>SNASDKGKLSLQDVAELIRARACQRVVVMVGAGISTPSGIPDFRSPGSGLYSNLQQYDLPYPEAIFELPFFFHNPKPFFTLAKELYPGNYKPNVTHYFLRLLHDKGLLLR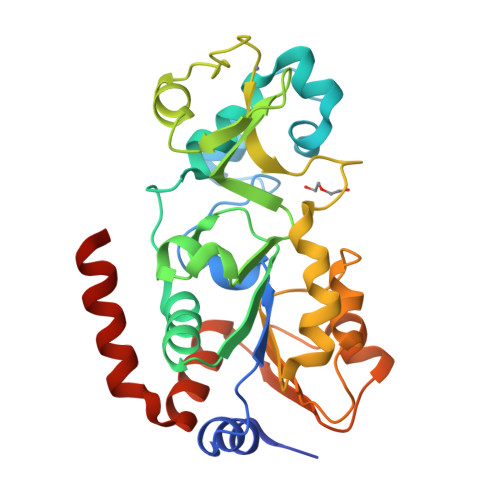LYTQNIDGLERVSGIPASKLVEAHGTFASATCTVCQRPFPGEDIRADVMADRVPRCPVCTGVVKPDIVFFGEPLPQRFLLHVVDFPMADLLLILGTSLEVEPFASLTEAVRSSVPRLLINRDLVGPLAWHPRSRDVAQLGDVVHGVESLVELLGWTEEMRDLVQRETGKLDGPDK[6x]> DREKIYQWINELSSPETRENALLELSKKRESVPDLAPMLWHSFGTIAALLQEIVNIYPSINPPTLTAHQSNRVCNALALLQCVASHPETRSAFLAAHIPLFLYPFLHTVSKTRPFEYLRLTSLGVIGALVKTDEQEVINFLLTTEIIPLCLRIMESGSELSKTVATFILQKILLDDTGLAYICQTYERFSHVAMILGKMVLQLSKEPSARLLKHVVRCYLRLS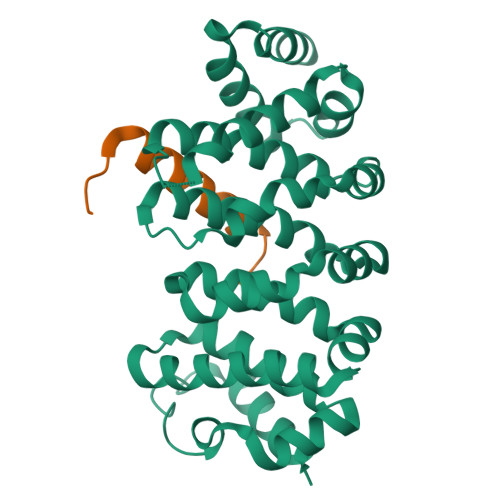DNPRAREALRQCLPDQLKDTTFAQVLKDDTTTKRWLAQLVKNLQ;> HMWETLDDQRALQLALDQLSLLGL> MDSSEDDGNKVAHLWPDPPAFWKDFTPENIERYNALKQTYA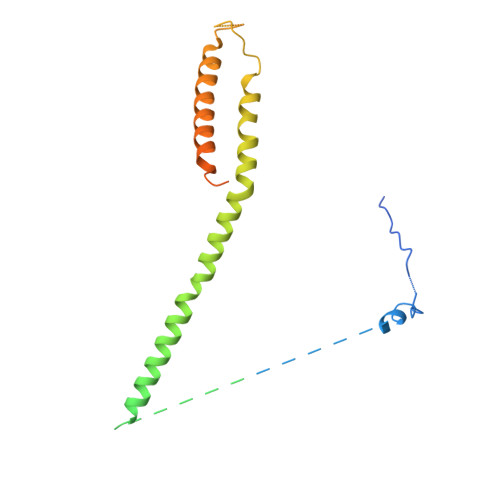QQHGLSSDALVRIPDVPADLINLQPPPEPVDGKWKLYGQQEALANSLQSLEDAGIQRLAPASETTSDSKHFDRGFELKKLAKSLLVNYLELMGIMSINPAHASEKVQDIKTIVLNFHHILNEYRPHQAREQLIQLMQDHLDAKRNETAAVRAVVDKAKRLIEGLASIEIPKVEDDNGRKAVEVERAALAERREIAAWQEADALFT> MNSTPIEEARSLLNPSNAPTRYAERSVGPFSLAAIWFAMAIQVAIFIAAGQMTSSFQVWQVIVAIAAGCTIAVILLFFTQSAAIRWGINFTVAARMPFGIRGSLIPITLKALLSLFWFGFQTWLGALALDEITRLLTGFTNLPLWIVIFGAIQVVTTFYGITFIRWMNVFASPVLLAMGVYMVYLMLDGADVSLGEVMSMGGENPGMPFSTAIMIFVGGWIAVVVSIHDIVKECKVDPNASREGQTKADARYATAQWLGMVPASIIFGFIGAASMVLVGEWNPVIAITEVVGGVSIPMAILFQVFVLLATWSTNPAANLLSPAYTLCSTFPRVFTFKTGVIVSAVVGLLMMPWQFAGVLNTFLNLLASALGPLAGIMISDYFLVRRRRISLHDLYRTKGIYTYWRGVNWVALAVYAVALAVSFLTPDLMFVTGLIAALLLHIPAMRWVAKTFPLFSEAESRNEDYLRPIGPVAPADESATANTKEQNGSENLYFQ

Mhp1 from the Gram-positive Microbacterium liquefaciens is an integral membrane protein that mediates the Na+-dependent binding and uptake of 5-aryl-substituted hydantoins (Suzuki & Henderson, 2006; Weyand et al, 2008). Mhp1 belongs to the nucleobase-cation-symport-1, NCS1, family of secondary active transporters (Weyand et al, 2008) found widely in bacteria, archaea (Ma et al, 2013), fungi and plants (Mourad et al, 2012; Witz et al, 2012; Schein et al, 2013). The structure of Mhp1 comprises twelve transmembrane helices (TMHs), which include the ten core TMHs characteristic of the superfamily with an additional two at the C-terminus (Weyand et al, 2008). The core can be divided into two motifs, a bundle motif (TMHs 1, 2, 6 and 7) and a hash motif (TMHs 3, 4, 8 and 9) (Shimamura et al, 2010).

The structure of Mhp1 in complex with L-5-(1H-indol-3-ylmethyl)hydantoin (L-IMH) was determined at 3.4 Å resolution. The L-IMH ligand is clearly defined in the electron density, residing between the bundle and hash motifs (Fig1A and B). L-IMH binds in a more extended conformation than was previously modelled for L-BH with the hydantoin ring reoriented by 180°. The hydantoin moiety mainly interacts with residues on the hash motif. It lies approximately parallel to the indole ring of Trp117 such that the two aromatic groups form a face-to-face π-stacking interaction and appears to be oriented by hydrogen bonding interactions with Asn318, Gln121 and Gly219 (Fig1B–D). This latter interaction with Gly219 at the breakpoint of TMH6 on the bundle was not apparent previously. The indole moiety of L-IMH packs between the main chain of Gly219 and the side chain of Gln42 at the breaks of the bundle helices TMH6 and TMH1, respectively, and forms an edge-to-face π-stacking interaction with Trp220 (Fig1B–D). Overall, this region of the Mhp1 protein forms a hydrophobic pocket that accommodates the indole moiety of the hydantoin as shown in the surface representation in Fig1C. Trp117 and Trp220 sandwich L-IMH in the binding pocket. In the IMH-Mhp1 crystal structure, there is very limited space available in the region of Gly219 such that substitution of this glycine with any other amino acid would result in a clash of the amino acid side chain with the indole ring of L-IMH.> MPSLMSFGSCQWIDQGRFSRSLYRNFKTFKLHEMHGLCMPNLLLNPDIHGDRIIFVCCDDLWEHDLKSGSTRKIVSNLGVINNARFFPDGRKIAIRVMRGSSLNTADLYFYNGENGEIKRITYFSGKSTGRRMFTDVAGFDPDGNLIISTDAMQPFSSMTCLYRVENDGINFVPLNLGPATHILFADGRRVIGRNTFELPHWKGYRGGTRGKIWIEVNSGAFKKIVDMSTHVSSPVIVGHRIYFITDIDGFGQIYSTDLDGKDLRKHTSFTDYYPRHLNTDGRRILFSKGGSIYIFNPDTEKIEKIEIGDLESPEDRIISIPSKFAEDFSPLDGDLIAFVSRGQAFIQDVSGTYVLKVPEPLRIRYVRRGGDTKVAFIHGTREGDFLGIYDYRTGKAEKFEENLGNVFAMGVDRNGKFAVVANDRFEIMTVDLETGKPTVIERSREAMITDFTISDNSRFIAYGFPLKHGETDGYVMQAIHVYDMEGRKIFAATTENSHDYAPAF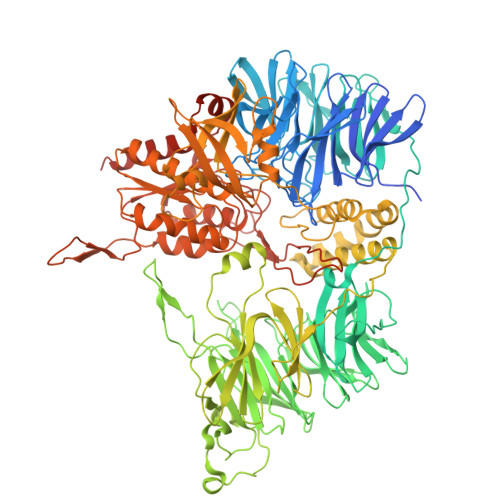DADSKNLYYLSYRSLDPSPDRVVLNFSFEVVSKPFVIPLIPGSPNPTKLVPRSMTSEAGEYDLNDMYKRSSPINVDPGDYRMIIPLESSILIYSVPVHGEFAAYYQGAPEKGVLLKYDVKTRKVTEVKNNLTDLRLSADRKTVMVRKDDGKIYTFPLEKPEDERTVETDKRPLVSSIHEEFLQMYDEAWKLARDNYWNEAVAKEISERIYEKYRNLVPLCKTRYDLSNVIVEMQGEYRTSHSYEMGGTFTDKDPFRSGRIACDFKLDGDHYVVAKAYAGDYSNEGEKSPIFEYGIDPTGYLIEDIDGETVGAGSNIYRVLSEKAGTSARIRLSGKGGDKRDLMIDILDDDRFIRYRSWVEANRRYVHERSKGTIGYIHIPDMGMMGLNEFYRLFINESSYQGLIVDVRFNGGGFVSQLIIEKLMNKRIGYDNPRRGTLSPYPTNSVRGKIIAITNEYAGSDGDIFSFSFKKLGLGKLIGTRTWGGVVGITPKRRLIDGTVLTQPEFAFWFRDAGFGVENYGVDPDVEIEYAPHDYLSGKDPQIDYAIDALIEELRNWNEELPQRPS4'-fluoro-4,5-dihydroxy-N-{(2E)-3-[(2S,4R,5R)-4-hydroxy-5-(6-methyl-9H-purin-9-yl)tetrahydrofuran-2-yl]prop-2-en-1-yl}biphenyl-3-carboxamide 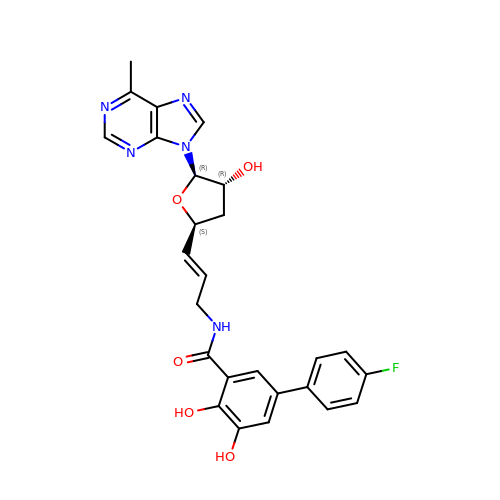| C26 H24 F N5 O5 | NFOSSDOJFGCEOO-DEAZYUCPSA-N> GSTGSMPCPKEDTPNSVWEPAKAKYVFRDVVQITCLDGFEVVEGRVGATSFYSTCQSNGKWSNS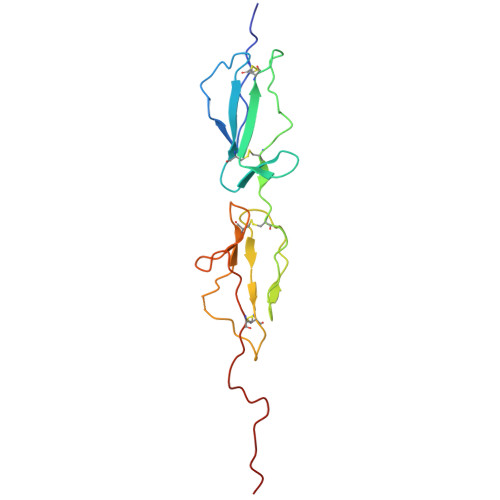KLKCQPVDCGIPESIENGKVEDPESTLFGSVIRYTCEEPYYYMENGGGGEYHCAGNGSWVNEVLGPELPKCVPVCGVPREPFEEKQR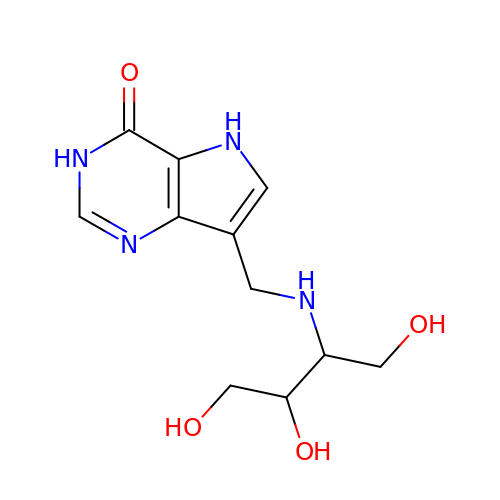7-({[(1R,2S)-2,3-DIHYDROXY-1-(HYDROXYMETHYL)PROPYL]AMINO}METHYL)-3,5-DIHYDRO-4H-PYRROLO[3,2-D]PYRIMIDIN-4-ONE | C11 H16 N4 O4 | CGYSFECPLYEOMH-HTQZYQBOSA-N Recruitment of Pol III to these genes requires the essential transcription factors TFIIIB and TFIIIC2. The six subunits of yeast TFIIIC are partitioned into two DNA-binding subcomplexes (τA and τB). The binding of these intragenic promoters by TFIIIC permits the assembly of TFIIIB, upstream of the transcription start site, which subsequently leads to the recruitment of Pol III, the formation of a PIC and finally to transcription. A genetic study suggests that the two largest TFIIIC subunits, τ138 and τ131, are responsible for connecting τA and τB16.

Given that our crosslinking data implicated the TPR array of τ131 in connecting τA and τB, and the reported importance of this region for TFIIIB assembly, we determined the crystal structure of the TPR array (residues 123–566) in two different space groups (P62 and P43). Starting from a construct expressing residues 1–580 of τ131, we identified a stable fragment by limited proteolysis and mass spectrometry corresponding to residues 123–566. We were able to collect diffraction data up to 3.15 Å (P62) and 3.4 Å (P43) resolution. The lower-resolution structure was solved by multiple isomorphous replacement with anomalous signal (MIRAS), using anomalous signal from crystals prepared with selenomethionine substituted proteins or native crystals soaked with p-chloromercuribenzensulfonic acid to final Rwork/Rfree values of 20.9%/24.5% The higher-resolution structure was solved using selenomethionine substituted protein in single anomalous dispersion (SAD) experiments and subsequently refined to Rwork/Rfree values of 25.0%/28.7%. The structure reveals the presence of 10 TPR repeats, while only nine TPR repeats had been predicted. Rather than forming an extended super-helix, the TPR array is instead separated into two ‘arms' by a central region that contains an extended helix and a disordered coil we call ‘ring' domain. This insertion causes a bend in the TPR array, positioning the TPRs of the right arm closer to the TPRs of the left arm. A superimposition of the two crystal forms and an analysis of temperature factors reveal flexibility at TPRs 1–3, 8–10 and residues at the extremes of the extended helix. Despite crystal contacts in these regions, the accommodation of the TPR array in these arrangements in two different crystal forms suggests that the conformational changes are indeed permitted within the TPR array.

> GAMVLDPEVAQLLSQANEAFVRNDLQVAERLFNEVIKKDARNFAAYETLGDIYQLQGRLNDCCNSWFLAAHLNASDWEFWKIVAILSADLDHVRQAIYCFSRVISLNPMEWESIYRRSMLYKKTGQLARALDGFQRLYMYNPYDANILRELAILYVDYDRIEDSIELYMKVFNANVERREAILAALENALDSSDEESAAEGEDADEKEPLEQDEDRQMFPDINWKKIDAKYKCIPFDWSSLNILAELFLKLAVSEVDGIKTIKKCARWIQRRESQTFWDHVPDDSEFDNRRFKNSTFDSLLAAEKEKSYNIPIDIRVRLGLLRLNTDNLVEALNHFQCLYDETFSDVADLYFEAATALTRAEKYKEAIDFFTPLLSLEEWRTTDVFKPLARCYKEIESYETAKEFYELAIKSEPDDLDIRVSLAEVYYRLNDPETFKHMLVDVVEMR tert-butyl 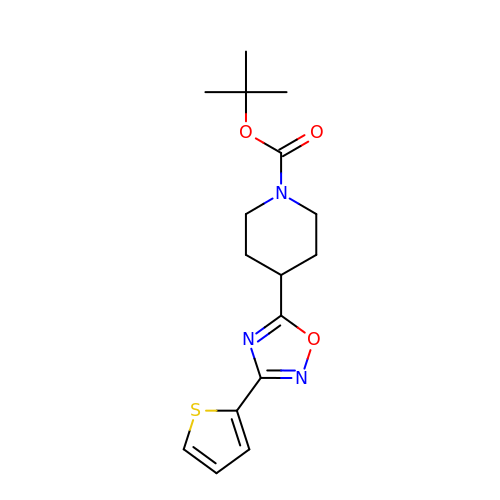4-(3-thiophen-2-yl-1,2,4-oxadiazol-5-yl)piperidine-1-carboxylate | C16 H21 N3 O3 S | METBQPRXNZHZMB-UHFFFAOYSA-N>[2x]HHHHHHMIVLFVDFDYFYAQVEEVL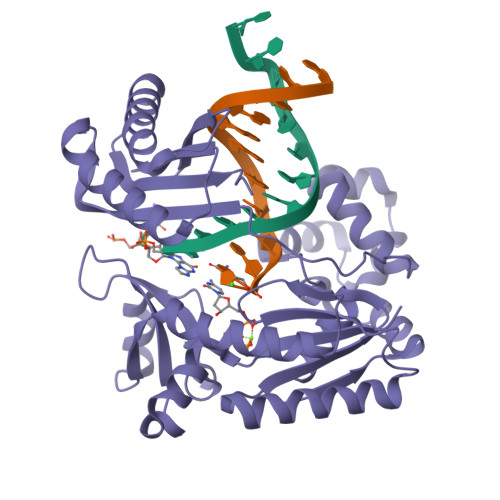NPSLKGKPVVVCVFSGRFEDSGAVATANYEARKFGVKAGIPIVEAKKILPNAVYLPMRKEVYQQVSSRIMNLLREYSEKIEIASIDEAYLDISDKVRDYREAYNLGLEIKNKILEKEKITVTVGISKNKVFAKIAADMAKPNGIKVIDDEEVKRLIRELDIADVPGIGNITAEKLKKLGINKLVDTLSIEFDKLKGMIGEAKAKYLISLARDEYNEPIRTRVRKSIGRIVTMKRNSRNLEEIKPYLFRAIEESYYKLDKRIPKAIHVVAVTEDLDIVSRGRTFPHGISKETAYSESVKLLQKILEEDERKIRRIGVRFSKFIE>[2x]GKITFYEDRGFQGRHYECSTDHSNL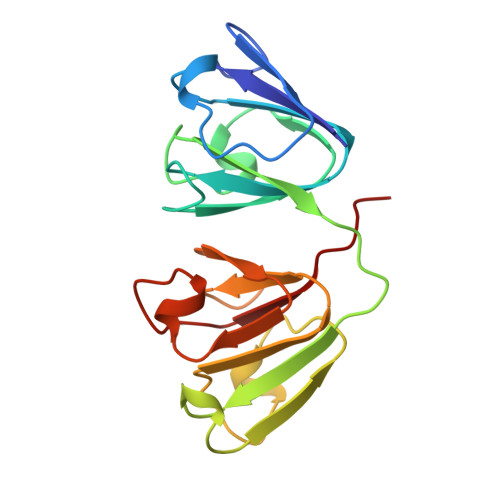QPYFSRCNSVRVDSGCWMLYEQPNFTGCQYFLRRGDYPDYQQWMGFSDSVRSCRLIPHSSSHRIRIYEREDYRGQMVEITDDCPHLQDRFHFSDFHSFHVMEGYWVLYEMPNYRGRQYLLRPGEYRRYHDWGAMNARVGSLRRIMDFY>LHRNSLIVLADVALFLALYHFLPFEHNVVLGISMLAFIAVLWLTEALHVTVTAILVPVMAVFFGIFETQAALNNFANSIIFLFLGGFALAAAMHHQGLDKVIADKVLAMAQGKMSVAVFMLFGVTALLSMWISNTATAAMMLPLVLGVLSKVDADKQRSTYVFVLLGVAYSASIGGIATLVGSPPNAIAAAEVGLSFTDWMKFGLPTAMMMLPMAIAILYFLLKPTLNGMFELDRAPVNWDKGKVVTLGIFGLTVFLWIFSSPINAALGGFKSFDTLVALGAILMLSFARVVHWKEIQKTADWGVLLLFG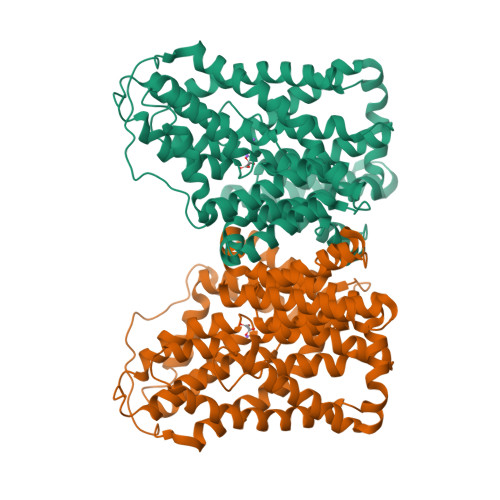GGLCLSNVLKQTGTSVFLANALSDMVSHMGIFVVILVVATFVVFLTEFASNTASAALLIPVFATVAEAFGMSPVLLSVLIAVAASCAFMLPVATPPNAIVFASGHIKQSEMMRVGLYLNIACIGLLTAIAMLFWQ[4x]> MGSSHHHHHHSSGRENLYFQGMQT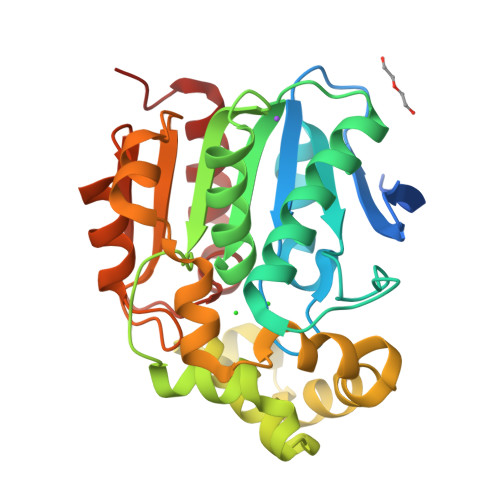SNIQTGSFNTFLNEAGTDKDTSILLLHGSGPGANAMSNWQYALPFLAENYHCLAPDIAGFGLSQHNCPPNGTSHWIDIWVQQQIDLLDAKGIEQTHIVGNSMGGGVTLHLLNRHPERFKKAVLMGPVGAPFAPTEGLTKGWEFYKDPSKEALEYLITKFLFDPSLLGNDIASIAAQRFDNVMKDEVRLQFEAMFSGGTKKGIDAFVLSDDELNNISHQMLVTHAREDFFIPLNNAYYLIDRIPNAQLHVFDHCGHWVQIEKKKAFNNLTKLFFDGMFDD> MASMTGGQQMGRDQAGITGTWYNQLGSTFIVTAGADGALTGTYESAVGNAESRYVLTGRYDSAPATDGSGTALGWTVAWKNNYRNAHSATTWSGQYVGGAEARINTQWLLTSG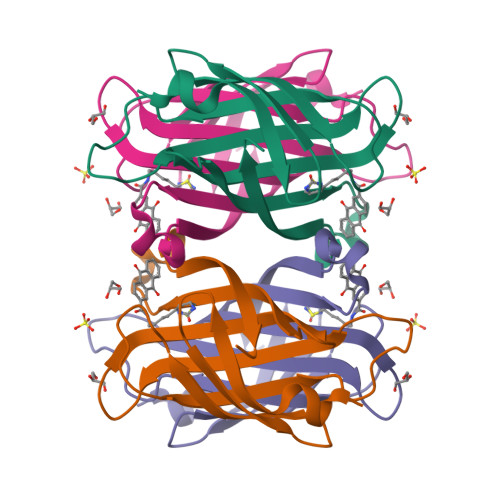TTEANAWKSTLVGHDTFTKVKPSAASIDAAKKAGVNNGNPLDAVQQ>[2x]TTPSMEDY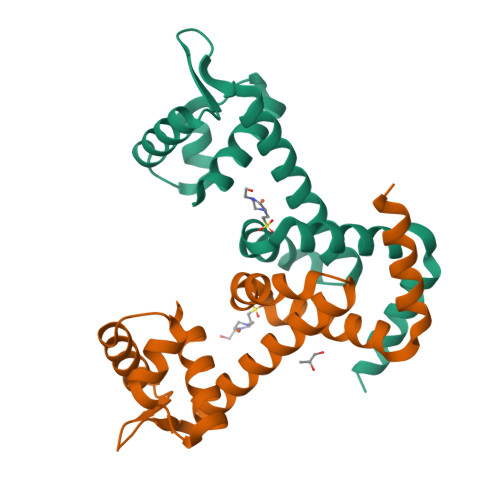IEQIYMLIEEKGYARVSDIAEALAVHPSSVTKMVQKLDKDEYLIYEKYRGLVLTSKGKKIGKRLVYRHELLEQFLRIIGVDEEKIYNDVEGIEHHLSWNSIDRIGDLVQYFEEDDARKKDLKSIQKKTEHHNQ>GPGSMTRREQDSLGERDIPMDAYFGIQTLRAVENFSLSDVALNHIPALVRALAMVKKAAATANYKLRQLPEPKYAAIVAACDDIIDGLLMEQFVVDVFQGGAGTSSNMNANEVIANRALEHLGRPRGDYQTIHPNDDVNMSQSTNDVYPTAVRLALLLSQNQVQTALHRLIAAFEAKGREFATVIKIGRTQLQDAVPITLGQEFEAFAATLREDTARLEEVAALFREVNLGGTAIGTRINASHAYAEQAIVELSQISGIELKATGNLVEASWDTGAFVTFSGILRRIAVKLSKIANDLRLLSSGPRSGLGEIRLPAVQPGSSIMPGKVNPVIPESVNQVCYQVIGNDLTVTMAAESGQLQLNAFEPLIVYNILSSMRLLGRAMTNLAERCVDGIEANVERCRAGAEESISLATALVPVVGYARAAEIAKQALASGQTVMEVAISKGLDASALTIMLDPLR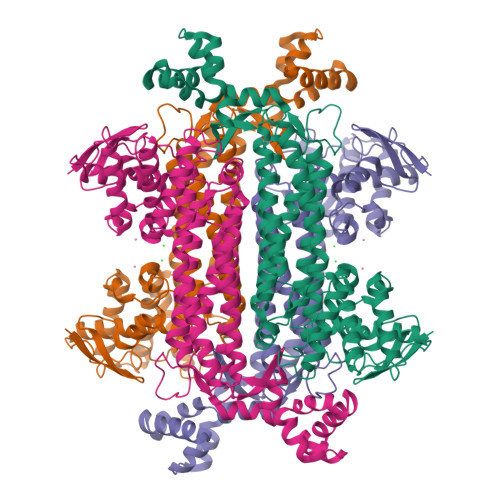MAFPPETHDKEAHH[4x]>GPHADGDQNLFDYQFTGTPEEPIKGYWTTTISYRDSKPKISLTIRQEFVEGGVESQAVLATVVGRPHLQDFLLLKRKHLEYSDYPESIDL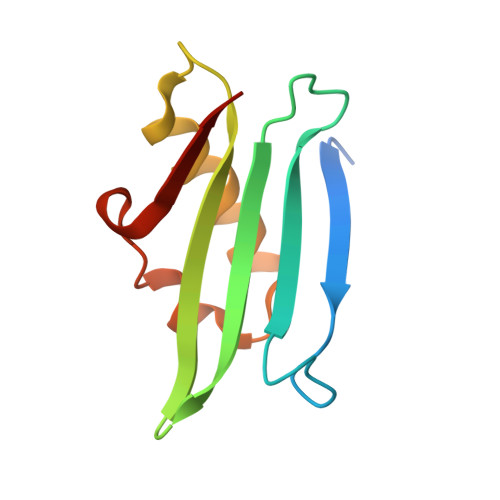IEFGDVKVIEKTV[2x]>[2x]MHHHHHHNLALNKTATASSIEGAGFEASRAFDGSSTTRWASAEGVDPQWIYVNLGSSQ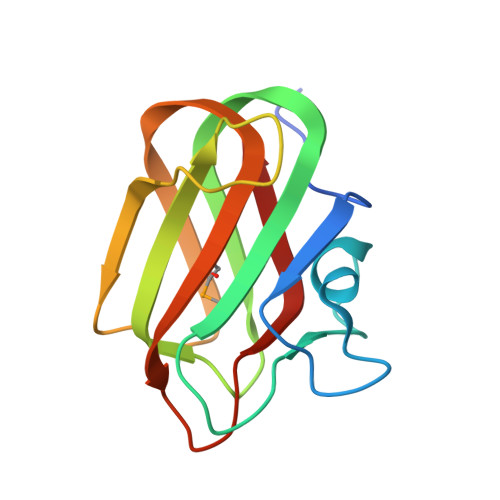TVNRVKLNWEAAYASSYTIQVSNDSGTPTNWTTVYTTTTGDGGIDDITFTARTAKYVRMHGTVRGTPYGYSLWEFEVYG>[2x]MTQFTDIDKLAVSTIRILAVDTVSKANSGHPGAPLGMA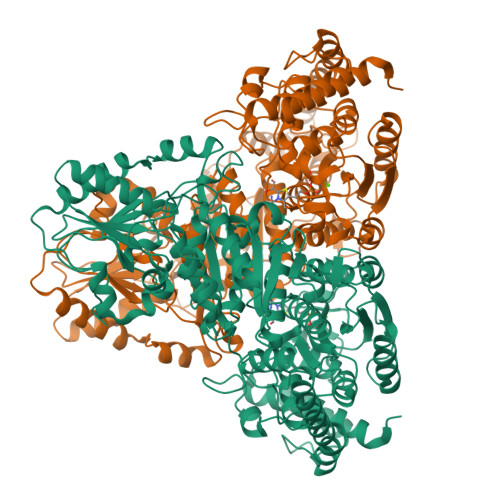PAAHVLWSQMRMNPTNPDWINRDRFVLSNGHAVALLYSMLHLTGYDLSIEDLKQFRQLGSRTPGHPEFELPGVEVTTGPLGQGISNAVGMAMAQANLAATYNKPGFTLSDNYTYVFLGDGCLQEGISSEASSLAGHLKLGNLIAIYDDNKITIDGATSISFDEDVAKRYEAYGWEVLYVENGNEDLAGIAKAIAQAKLSKDKPTLIKMTTTIGYGSLHAGSHSVHGAPLKADDVKQLKSKFGFNPDKSFVVPQEVYDHYQKTILKPGVEANNKWNKLFSEYQKKFPELGAELARRLSGQLPANWESKLPTYTAKDSAVATRKLSETVLEDVYNQLPELIGGSADLTPSNLTRWKEALDFQPPSSGSGNYSGRYIRYGIREHAMGAIMNGISAFGANYKPYGGTFLNFVSYAAGAVRLSALSGHPVIWVATHDSIGVGEDGPTHQPIETLAHFRSLPNIQVWRPADGNEVSAAYKNSLESKHTPSIIALSRQNLPQLEGSSIESASKGGYVLQDVANPDIILVATGSEVSLSVEAAKTLAAKNIKARVVSLPDFFTFDKQPLEYRLSVLPDNVPIMSVEVLATTCWGKYAHQSFGIDRFGASGKAPEVFKFFGFTPEGVAERAQKTIAFYKGDKLISPLKKAF>[2x]MTLGTNQVSKTHSFMTVSLIELWERFGYYGMQALIVYFMVQRLGFDDSRANLV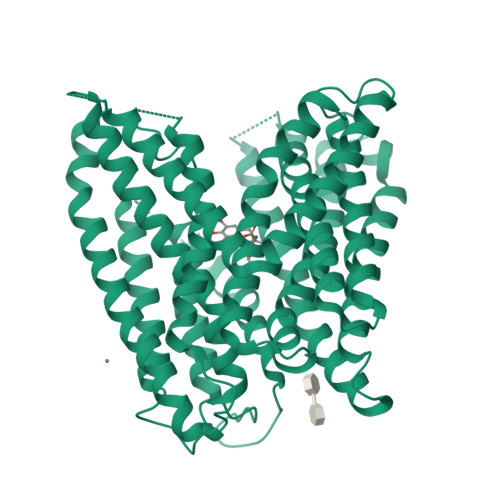WSACAALIYVSPAIGGWVGDKILGTKRTMLLGAGILSVGYALMTVPTENTWFMFSALGVIVVGNGLFKPNAGNLVRKIYEGDDSKIDSAFTIYYMAVNVGSTFSMLLTPWIKDYVNAQYGNEFGWHAAFAVCCVGILVGLGNYALMHKSLANYGSEPDTRPVNKKSLAIVLALAALSVVASAIILEYEDVARVFVYAAGVAVLGIFFHLIRTSEPSERAGLIAALILTVQTVFFFIFYQQMSTSLALFALRNVDWDFQVFGTHLWTWSPAQFQALNPIWIMVLSPVLAWSYSWAGRNNKDFSIAAKFALGFAVVAIGFFIYGFAGQFAVNGKTSSWVMIWGYASYSLGELLVSGLGLAMIARYVPARMGGFMMGAYFVASGISQYLGGVVANFASVPQDLVDPLQTLPVYTNLFNKLGVAAVVCTIIALAVLPLMRRLTESHHAHSSIENNAAASLRDVKAEQAENLYFQ;> AYA> GSMAASDEVNLIESRTVVPLNTWVLISNFKVAYNILRRPDGTFNRHLAEYLDRKVTANANPVDGVFSFDVLIDRRINLLSRVYRPAYADQEQPPSILDLEKPVDGDIVPVILFFHGGSFAHSSANSAIYDTLCRRLVGLCKCVVVSVNYRRAPENPYPCAYDDGWIALNWVNSRSWLKSKKDSKVHIFLAGDSSGGNIAHNVALRAGESGIDVLGNILLNPMFGGNERTESEKSLDGKYFVTVRDRDWYWKAFLPEGEDREHPACNPFSPRGKSLEGVSFPKSLVVVAGLDLIRDWQ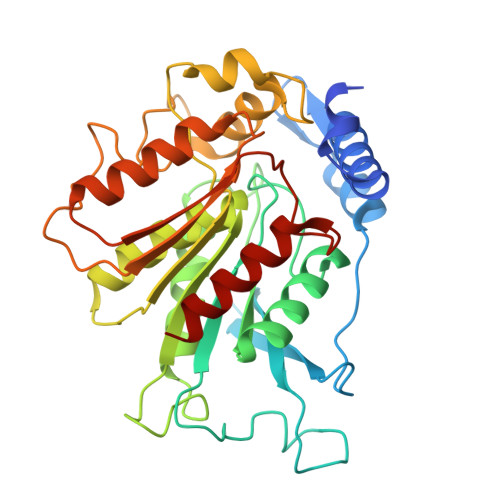LAYAEGLKKAGQEVKLMHLEKATVGFYLLPNNNHFHNVMDEISAFVNAEC> MEVRNMVDYELLKKVVEAPGVSGYEFLGIRDVVIEEIKDYVDEVKVDKLGNVIAHKKGEGPKVMIAAHMDQIGLMVTHIEKNGFLRVAPIGGVDPKTLIAQRFKVWIDKGKFIYGVGASVPPHIQKPEDRKKAPDWDQIFIDIGAESKEEAEDMGVKIGTVITWDGRLERLGKHRFVSIAFDDRIAVYTILEVAKQLKDAKADVYFVATVQEEVGLRGARTSAFGIEPDYGFAIDVTIAADIPGTPEHKQVTHLGKGTAIKIMDRSVICHPTIVRWLEELAKKHEIPYQLEILLGGGTDAGAIHLTKAGVPTGALSVPARYIHSNTEVVDERDVDATVELMTKALENIHELKI

We apply the integrated NMR/EM approach to the dodecameric 12 × 39 kDa (468 kDa) large aminopeptidase enzyme TET2 from Pyrococcus horikoshii which forms a large hollow lumen encapsulating 12 peptidase active sites. The dodecameric assembly forms a tetrahedral structure with ca. 12 Å wide openings, one on each of the four tetrahedron faces, providing access to the ca. 50 Å wide catalytic lumen. NMR and EM thus provided structural information about TET2 on very different length scales, but neither of the two techniques by themselves allowed to determine the structure at the atomic scale, owing to the lack of long-range distance information in NMR, and the inability to build a robust model from the EM map.

We use cryo-EM maps with resolutions of 4.1, 6, and 8 Å (the latter two were obtained by Fourier-space truncation), as well as secondary structure and distance information from MAS NMR and solution-NMR. Despite its large subunit size of 353 residues, larger than any protein assigned to date by MAS NMR, we achieved a near-complete NMR resonance assignment in a reliable manner, which allows the residue-wise determination of the backbone conformation, as well as hundreds of experimental distance restraints involving the protein backbone and side chain methyl groups, but by themselves these data are insufficient for structure determination. An automated approach that jointly exploits the EM map, NMR secondary structure, and distance restraints is presented, that allowed us to obtain the structure of TET2 at a backbone root-mean-square-deviation (RMSD), of 0.7 Å to the crystal structure. In the first step, after detection of the α-helices in the EM map and in the sequence, the various possibilities of placing α-helical sequence stretches into α-helix density features are systematically and combinatorially tested, performing with each of these helix-to-density assignments a restrained-MD type structure calculation with CYANA. Subsequently, the correct helix-to-density assignment is identified through objective criteria that compare the resulting structural models to experimental NMR and EM observables. The refinement stage of the protocol, an automated iterative procedure denoted here as step 2, consists of iterative cycles of (i) a flexible fitting of the initial structure into the 8 Å EM density with iMODFIT26, and (ii) CYANA structure calculations. In step 3, a real-space structure refinement was applied in the XPLOR-NIH software, using the full Coulombic potential map, first at 8 Å, then at 6 Å and lastly at 4.1 Å resolution, and all NMR restraints, calculating the full dodecamer. Figure 3 shows the evolution of the structure from the initial model to the final structure, which was obtained with high precision (bundle backbone RMSD over the 20 lowest-energy structures of 0.29 Å for one subunit).> SNAMKLIAIDL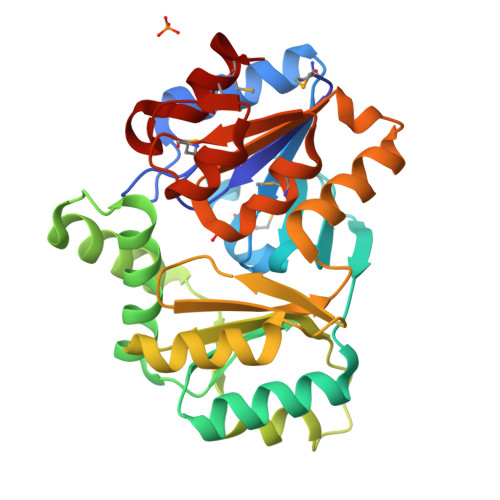DGTLLNSKHQVSLENENALRQAQRDGIEVVVSTGRAHFDVMSIFEPLGIKTWVISANGAVIHDPEGRLYHHETIDKKRAYDILSWLESENYYYEVFTGSAIYTPQNGRELLDVELDRFRSANPEADLSVLKQAAEVQYSQSGFAYINSFQELFEADEPIDFYNILGFSFFKEKLEAGWKRYEHAEDLTLVSSAEHNFELSSRKASKGQALKRLAKQLNIPLEETAAVGDSLNDKSMLEAAGKGVAMGNAREDIKSIADAVTLTNDEHGVAHMMKHLL IL18 is a pro-inflammatory cytokine belonging to the interleukin 1 superfamily and plays an important role in both innate and acquired immune responses by inducing interferon-γ (IFN-γ) production from T lymphocytes and macrophages while also enhancing the cytotoxicity of natural killer cells. Mammals and poxviruses encode homologous inhibitory proteins of IL18, named IL18BPs, which regulate IL18 activity and, in the case of the viral proteins, contribute to virulence. To understand the mechanism by which yatapoxvirus IL18BPs neutralize IL18, we solved the high-resolution crystal structure of the Yaba-Like Disease Virus (YLDV) IL18BP:IL18 complex. The structure of the complex shows that the YLDV-IL18BP forms a homo-dimer in a back-to-back fashion, with each protomer binding to a molecule of IL18, forming a hetero-tetramer complex with a stoichiometry of 2∶2.

Furthermore, a crystal from the complex of IL18 (8S) and a three-cysteine mutant of YLDV-IL18BP (ΔC21, C87S, C132S) diffracted to 1.75 Å. The two structures are essentially identical to each other with a root mean square deviation (r.m.s.d) of less than 0.4 Å, and the three mutated cysteines in YLDV-IL18BP are distant from the IL18 binding interface. Therefore, for discussion of protein:protein interactions between YLDV-IL18BP and IL18, we will mainly focus on the higher resolution structure of the mutant YLDV-IL18BP. In the triple-cysteine mutant YLDV-IL18BP:IL18 structure, the βE–βF loop is not visible in the electron density map, suggesting that C21–C87 SS bond stabilizes the local structure, particularly the βE–βF loop. However, the C21–C87 SS bond is not critical for the overall structure of YLDV-IL18BP or its binding with IL18 (shown later). The homo-dimer interface involves mainly βA, βB, βH and the C-terminal helix H3. It involves extensive hydrophobic interactions in the center (I29, H30, V31, P32 and V33 from βA, the aliphatic side chain of E122, V124 from βH and I129 from H3) flanked by hydrogen bonding and charge-charge interactions, burying approximately 1,700 Å2 and 1,465 Å2 solvent accessible surface area (ASA) for the wild-type complex and the triple-cysteine mutant complex, respectively. The lack of the C132-C132 SS bond in the triple-cysteine mutant complex caused the disorder of four residues at the C-terminus beyond S132, resulting in a slightly smaller ASA. However, the triple-cysteine mutant of YLDV-IL18BP displays nearly identical structure as the WT protein, and it exists as a dimer in solution judging by size exclusion chromatography and dynamic light scattering analysis (data not shown). Therefore, the dimerization is not solely dependent on the C132-C132 inter-chain SS bond.

>MVKTRSVNIHVPVKETSKVVLECRGDSYFRHFSYVYWIIGKNKTVDQLPPNSGYRERIYLFKKPHRSENRPRADLILTNITDEMRNEKLTCVLIDPKDPLKESVILSKIWNSVYKI[2x];>[2x]YFGKLESKLSVIRNLNDQVLFIDQGNRPLFEDMTDSDSRDNAPRTIFIISMYKDSQPRGMAVTISVASAAASTLSSENKIISFKEMNPPDNIKDTKSDIIFFQRSVPGHDNKMQFESSSYEGYFLASEKERDLFKLILKKEDELGDRSIMFTVQNED> MPRVRPLGPNPQDRPNWDSMNDGQRRYAMEQWNLARVRRGEYFDPPGDDDLPLTQADAIDNFDLDLLGSPQEAEQPSQQSEDGVDDFLQQVRDRQDLRDAGPSNAPQPNMADVEMAQVSSSSSGSKRGSDGSGPPSKVSKSGTSLPGTGGNLDGMARGGSGEGGATAILRPIGLHVEKFQQTYRKKWRFLTSANANVILAEAASGERPARWALTTGMASIPWEYLFFYMSPAEYNRMKNYPGTFAKSASVRIRTWNTRVAFQTGDTQTANATLNQNKFLQVAKGIRSIPFICSTNRKYTYSDTEPMQPTGFATLTSYEYRDGLKIAMYGYDNDSPDFAKKP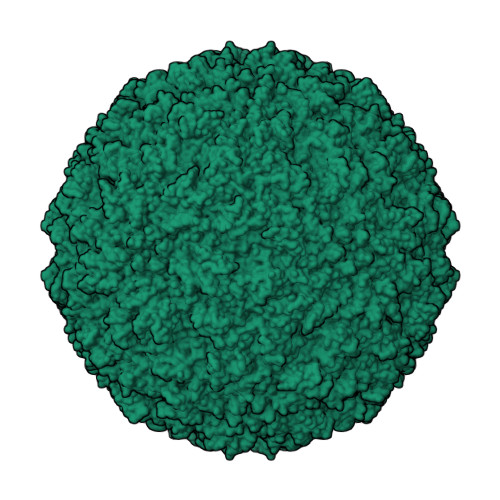PADATGAEIYLQDYLTIYTNDARATTGTKILAGFPPYKNFIEEFDASACINTDVVAMDYDFSYAPLVPQFAPVPNNLITQNYNASYPAGTKNEVTAAKTTDSSQATPPTQVRNAPRKYIQGPNADTTFFDEEQNYLRVPIEQGGIFEEVNVETVHDTQMPSINVGIRAVPKLTTIDETTQANSWLDAQGYFEVDCVLTTESVDPYTYIKGGCYSANTKSQLQYFANDGRPIAKVYDNPNVYGRMQMIKTVKP>[3x]MAHHHHHHMFRTHTNGELSLKNLNEEVTLSGWVQTIRDKGFMIWIDLRDRYGITQLVFDQDRSSAALLEEAKKLGREFVIQVSGKVIERASKNPKIPTGEIEILVEKLTILNNSELPPFTIEDETDGGEELRMKYRYLDIRRNPVKEKLIFRHKIAQKVRNYLSDQGFIEVETPVLIKSTPEGARDFVVPSRMNPGQFYALPQSPQTFKQLLMVGGMDKYFQIVKCFRDEDLRADRQPEFTQIDCE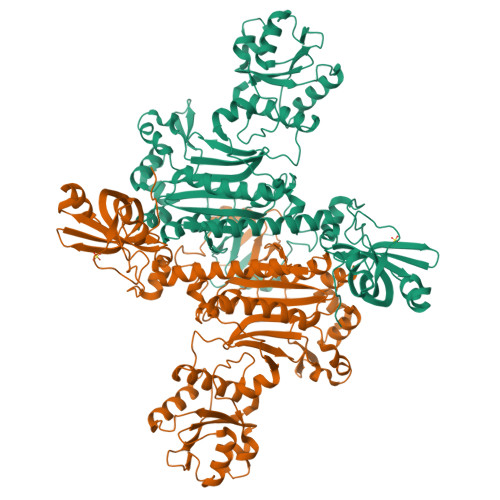MAFVEQEDVMNIFEGLTQNLLKDIAGQEFGKFPRMTFAEAMKKYGNDKPDIRFGMEFHELNDLVKGKDFKIFDEAELVVGINVEGCAEYTRKQIDELTDWIKRPQIGATGMVWIKYQADGIVTSSVNKFYNEEDLKKIAEEFGAKPGDLMLVLSGNENKVRAQLSALRMELGNRLGLRKGNEFAPLWVIDFPLLEWDEDTQRYHAMHHPFTSPKPEDIHLLENEAGKARANAYDLVINGNEIGGGSIRIFDKDLQAQMFSLLGFTPEEAEAQFGFLMNAFKYGAPPHGGLAFGFDRLVAVLDGNEVIRDYIAFPKNNSGRDVMIDAPASIANEQLDELALTININE> MDNVLPVDSDLSPNISTNTSEPNQFVQPAWQIVLWAAAYTVIVVTSVVGNVVVMWIILAHKRMRTVTNYFLVNLAFAEASMAAFNTVVNFTYAVHNEWYYGLFYCKFHNFFPIAAVFASIYSMTAVAFDRYMAIIHPLQPRLSATATKVVICVIWVLALLLAFPQGYYSTTETMPSRVVCMIEWPEHPNKIYEKVYHICVTVLIYFLPLLVIGYAYTVVGITLWASEGIDCSFWNESYLTGSRDERKKSLLSKFGMDEGVTFMFIGRFDRGQKGVDVLLKAIEILSSKKEFQEMRFIIIGKGDPELEGWARSLEEKHGNVKVITEMLSREFVRELYGSVDFVIIPSYFEPFGLV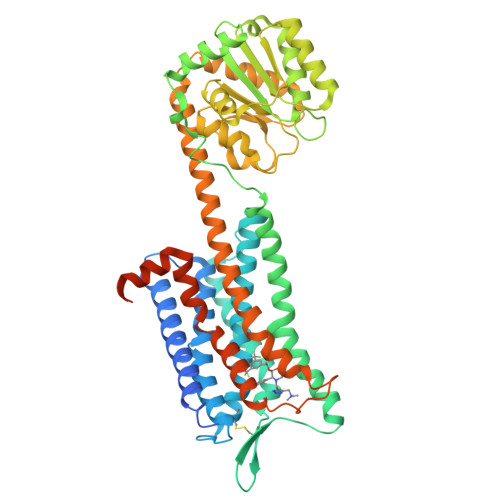ALEAMCLGAIPIASAVGGLRDIITNETGILVKAGDPGELANAILKALELSRSDLSKFRENCKKRAMSFSEQVSAKRKVVKMMIVVVCTFAICWLPFHIFFLLPYINPDLYLKKFIQQVYLAIMWLAMSSTMYNPIIYCCLNDRFRLGFKHAFRCCPFISAGDYEGLEMKSTRYLQTQGHHHHHHHHHH>[4x]GMELDDAYANGAYIEGAADYPPRWAASAEDFRNSLQDRARLNLSYGEGDRHKFDLFLPEGTPVGLFVFVHGGYWMAFDKSSWSHLAVGALSKGWAVAMPSYELCPEVRISEITQQISQAV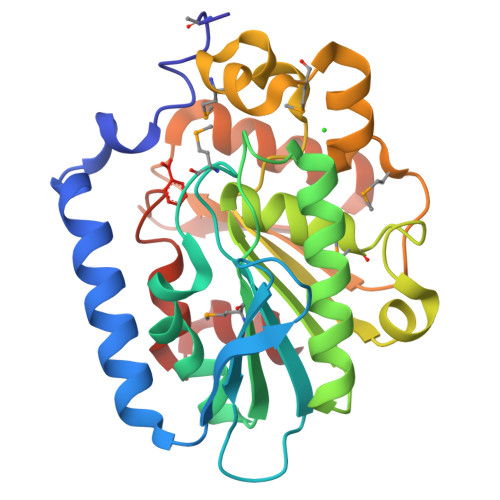TAAAKEIDGPIVLAGHSAGGHLVARMLDPEVLPEAVGARIRNVVPISPLSDLRPLLRTSMNEKFKMDADAAIAESPVEMQNRYDAKVTVWVGGAERPAFLDQAIWLVEAWDADHVIAFEKHHFNVIEPLADPESDLVAVITA>NAVCRGPGDKPTQNIQLFNGRYAIINNSTAYPSRNSISELKVPRDFVPSPGTFHGCSRFPSYSNHYGLWCYSHTVSNDTCDGSNPSVQILSVGKLITGDNGQPEHKTLYTQQLSQTDRLYHCSVTMTTLGCYILCSKPRVNETQDYETIGIEPMIIGMLGLDGVYTDLGNPVGISDNSLYAMYPGPGGGVMYKDFLVFPLHGGVRFSEASKMLGKNITFRGFPPSDTCTEHEKSLTQEPANMLTSPYYGEVLVLDFLYVCTLLDNIPGECSIQ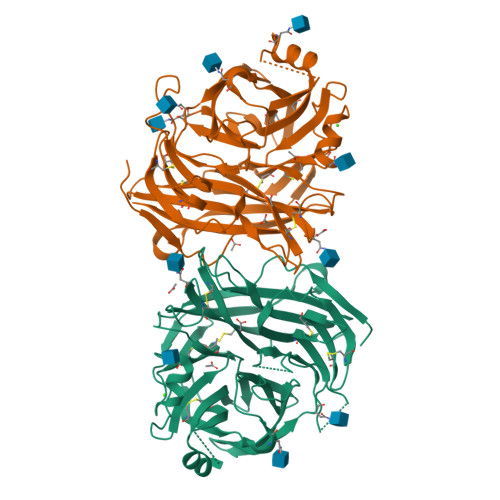LIPPDNMTMGSESKLYKLNNSLLLYKRSSSWWPYTEVYQLSLRVSKNSMKVRESVRLNITSTTRPGVEGCNINKVCPKVCVTGVFQAPGIIRKALSPKESNEDLLFFQAWTSDSIARQGPLISLCRADSCVLTIPLGNSDVFIGYTDSFCLSDRDNEKIYCVALLELDNMPYSEMTIRSFLYLIKGTETSQVAPA[2x]In this work, we employed an approach to disentangle noncovalent and hydrogen-bonding electric field changes during the reaction cascade of a multidomain protein, i.e., the phytochrome Agp2. Agp2 originates from Agrobacterium fabrum and carries a biliverdin (BV) chromophore. Phytochromes harbor a methine-bridged tetrapyrrole chromophore as a light-sensing unit, which upon light absorption undergoes a photoisomerization at the terminal methine bridge followed by a cascade of structural relaxations.18−21 This reaction sequence interconverts the parent states Pr and Pfr and involves proton translocation, which has been shown to be a prerequisite for the functional secondary structure transition of the tongue, a phytochrome-specific peptide segment. In the present work, we have generated two further variants with ortho-cyanophenylalanine (oCNF) at positions 165 or 192.

We determined the crystal structures of the Pfr state of Y165oCNF and F192oCNF variants with 1.90 and 2.06 Å resolution, respectively. For Y165oCNF, the residues Phe167 and Leu274 are slightly shifted away from the nearby oCNF165 by 0.9 and 0.8 Å, respectively, due to the larger space occupied by oCNF compared to the native Tyr165. Despite this minor difference, the BV chromophore structure remained unaffected by the Y165oCNF substitution, showing nearly perfect alignment with the WT Agp2-PCM. The region between 1500 and 1700 cm–1 is dominated by the C=C stretching modes of the methine bridges between pyrrole rings, which are particularly sensitive toward geometrical changes of the tetrapyrrole skeleton.54 In the Pfr state, a nearly perfect agreement between the WT and F192oCNF spectra in this region underpins the preservation of the chromophore structure in both proteins. This conclusion is largely valid also for Y165oCNF, although the stretching of the C–D methine bridge (C–D) displays a 4 cm–1 upshift, which suggests a slightly larger dihedral angle and thus stronger torsion of ring D than in the WT. Minor differences that do not affect the functional integrity include a slightly higher torsion of ring D and an increased keto content in the Pr state of Y165oCNF and the reaction kinetics. Interactions of the nitrile group in Y165oCNF seem to be more variable because the ortho position of the CN label allows for different, possibly coexisting rotamers. Our crystal structure of Y165oCNF in the Pfr state shows that H-bonding differs from that of the WT Agp2-PCM, as the nitrile group is pointing away from the potential H-bonding donors propC and H278 and no H-bonds are found except for a hydrogen bridge of the Y165oCNF backbone. Again, this finding is qualitatively in line with the nitrile stretching frequencies that are in each substate of Y165oCNF distinctly lower than in the Y165pCNF variant. In Y165oCNF, EF,tot remains largely constant within the accuracy of the field calculations, whereas in Y165pCNF, we note two extraordinarily high values in Lumi-F and Pr.

>[2x]MASTDYHVDLTNCDREPIHIPGYIQPHGCLIACDNAMRMVLRHSENCGELLGLEGDLNGRTAEDVLGKKLVHDLRNALTVTGRTTRPAMLPAMETSDGRSFDISLHRYKSTTIIEFEPSGSDAQPLGTARKMVDRIREADSVESLISRTTRLVKATLGYDRVMIXRFQEDGAGKVVSEAKQPELESFLGQYFPASDIPQQARALYLKNTLRIISDASGTRIPVLPAVDVSGEPLDLSYAHLRSVSPIHCEYLRNMGVAASMSISVIVDGALWGLIACHHYSPRVLSMPVRIAAEMFGEFFSMHLQVLKQKRRLDTINHAHAALDRFLRLAAHHANIEELLVDSFQDFADLMPCDGVGLWVGNNWHGHGATPPHDAIPRLARFVASASEGRVWATHALSQAIPEAEIYAGTAAGMLAIPLSQVKSDYLLFFRKEIVQNLNWAGNPEKSYETGPMGDRLTPRKSFAIWKETVRLQAQPWSEADREIAEAARIALVEVAFHHSEHHHHHH6-azidouridine 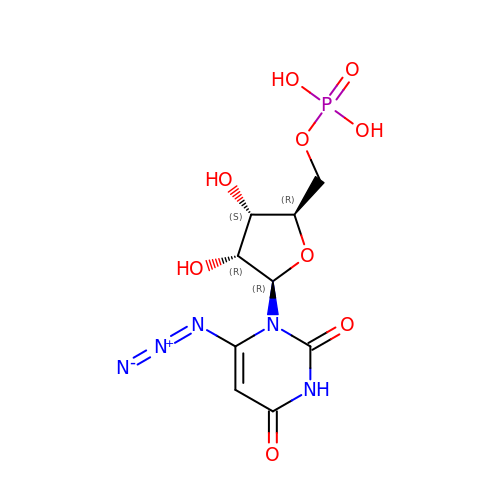5'-(dihydrogen phosphate) | C9 H12 N5 O9 P | GBBWDDPNGBRVEX-YXZULKJRSA-N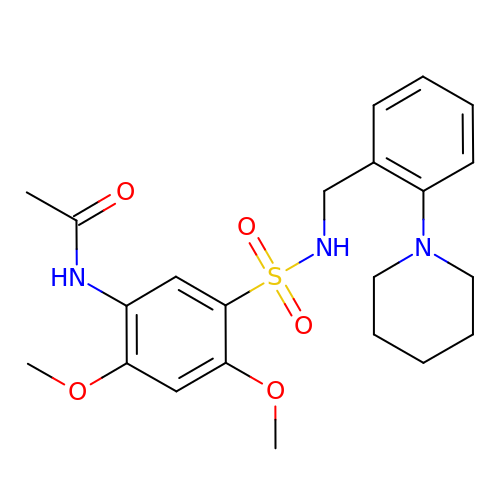N-{2,4-DIMETHOXY-5-[(2-PIPERIDIN-1-YLBENZYL)sulfamoyl]phenyl}acetamide | C22 H29 N3 O5 S | LDJDHSINBFNMFS-UHFFFAOYSA-N> MQHYLHIRPAPSDNLPLVDLIEHPDPIFDPKEKDLNETLLRSLLGGHYDPGFMATSPPEDRPGGGGGAAGGAEDLAELDQLLRQRPSGAMPSEIKGLEFSEGLAQGKKQRLSKKLRRKLQMWLWSQTFCPVLYAWNDLGSRFWPRYVKVGSCFSKRSCSVPEGMVCKPSKSVHLTVLRWRCQRRGGQRCGWIPIQYPIISECKCSC;> QAKHKQRKRLKSSCKRHPLYVDFSDVGWNDWIVAPPGYHAFYCHGECPFPLADHLNSTNHAIVQTLVNSVNSKIPKACCVPTELSAISMLYLDENEKVVLKNYQDMVVEGCGCR

pmcBone morphogenetic proteins (BMPs) are multifunctional cytokines belonging to the transforming growth factor-β (TGF-β) superfamily. BMP signaling occurs through binding to and subsequent oligomerization of two type I and two type II serine-threonine kinase receptors in the cell membrane, to form a heterohexameric complex. Finally, both Smad-dependent and Smad-independent signaling pathways are upregulated and downregulated by various cellular effectors, such as coreceptors and secreted antagonists. Thus, the former are membrane-bound proteins, known as auxiliary accessory receptors or coreceptors, which fine-tune signaling by promoting or inhibiting the interaction of BMP ligands to their authentic receptors, whereas the latter (e.g., Noggin and Gremlin) bind to BMP receptor recognition sites, hence physically preventing binding.

Crystals of the complex belong to the P6122 space group and allowed the structure to be solved at a resolution of 3.1 Å by using X-ray diffraction. Thus, Noggin covers around one-third of BMP-2 residues (i.e. 74 out of 228) and interacts through four large hydrophobic patches, 22 hydrogen bonds, and 2 ionic bonds in total. Finally, the overall structure reveals that Noggin masks both type 1 and 2 receptor-binding sites. Thus, the core of Noggin interacts with the type 2 receptor-binding site, while its N-terminal segment inserts into the type 1 receptor-binding site. The structure of the antagonist Noggin bound to BMP-2 reveals that the binding interface can be divided into three contact regions. Thus, a short hydrophobic segment (P35, A36, P37) of Noggin occupies the type 1 receptor-binding site of BMP-2, which consists of a large concave hydrophobic pocket. At the level of the type 2 receptor-binding interface, a concave hydrophobic structural element of Noggin, made up of six hydrophobic side chains (L43, L46, I47, I220, Y222, P223), interacts with two short convex hydrophobic segments of BMP-2 (i.e. V33 to P36 and V98 to L100). Finally, the third contact region involves a segment of BMP-2, which is located between the type 1 and type 2 receptor-binding sites. In this region of the BMP-2 structure, the N102 residue seems to play a key role in stabilizing the complex because it is involved in four hydrogen bonds (i.e. three with the amide side-chain group and one with the backbone carbonyl) with Noggin. Moreover, residues from 84 to 141, which are part of the dimerization interface, and residues from 209 to 213, which form a loop connecting strands β3 and β4, are not defined in our structure, probably as a result of their high flexibility.>[4x]MHHHHHHSSGRENLYFQGMEELIPLVNRLQDAFSALGQSCLLELPQIAVVGGQSAGKSSVLENFVGRDFLPRGSGIVTRRPLVLQLITSKAEYAEFLHCKGKKFTDFDEVRLEIEAETDRVTGMNKGISSIPINLRVYSPHVLNLTLID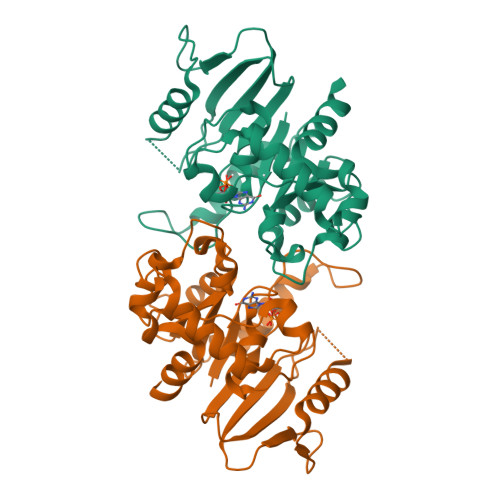LPGITKVPVGDQPPDIEYQIREMIMQFITRENCLILAVTPANTDLANSDALKLAKEVDPQGLRTIGVITKLDLMDEGTDARDVLENKLLPLRRGYVGVVNRSQKDIDGKKDIKAAMLAERKFFLSHPAYRHIADRMGTPHLQKVLNQQLTNHIRDTLPNFRNKLQGQLLS>[8x]MSQQPGVLPENMKRYMGRDAQRMNILAGRIIAETVRSTLGPKGMDKMLVDDLGDVVVTNDGVTILREMSVEHPAAKMLIEVAKTQEKEVGDGTTTAVVVAGELLRKAEELLDQN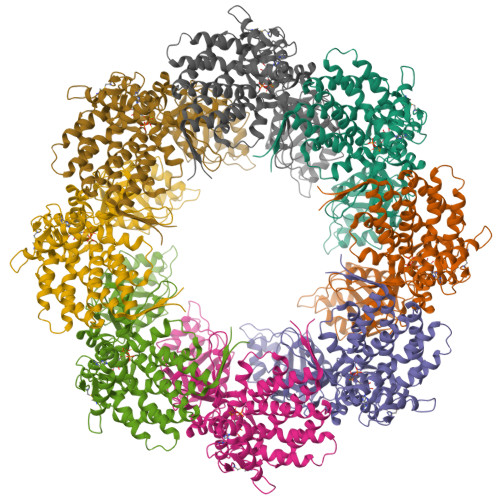VHPTIVVKGYQAAAQKAQELLKTIACEVGAQDKEILTKIAMTSITGKGAEKAKEKLAEIIVEAVSAVVDDEGKVDKDLIKIEKKSGASIDDTELIKGVLVDKERVSAQMPKKVTDAKIALLNCAIEETASEMLKDMVAEIKASGANVLFCQKGIDDLAQHYLAKEGIVAARRVKKSDMEKLAKATGANVITNIKDLSAQDLGDAGLVEERKISGDSMIFVEECKHPKAVTMLIRGTTEHVIEEVARAVDDAVGVVGCTIEDGRIVSGGGSTEVELSMKLREYAEGISGREQLAVRAFADALEVIPRTLAENAGLDAIEILVKVRAAHASNGNKCAGLNVFTGAVEDMCENGVVEPLRVKTQAIQSAAESTEMLLRIDDVIAAEKLRGAPDMGDMGGMPGMGGMPGMM> HMGFRWKLAHFRYLCQSNALPSHVKINVSRQTLFEDSFQQIMALKPYDLRRRLYVIFRGEEGLDYGGLAREWFFLLSHEVLNPMYCLFEYAGKNNYCLQINPASTINPDHLSYFCFIGRFIAMALFHGKFIDTGFSLPFYKRMLSKKLTIKDLESIDTEFYNSLIWIRDNNIEECGLEMYFSVDMEILGKVTSHDLKLGGSNILVTEENKDEYIGLMTEWRFSRGVQEQTKAFLDGFNEVVPLQWLQYFDEKELEVMLCGMQEVDLADWQRNTVYRHYTRNSKQIIWFWQFVKETDNEVRMRLLQFVTGTCRLPLGGFAELMGSNGPQKFCIEKVGKDT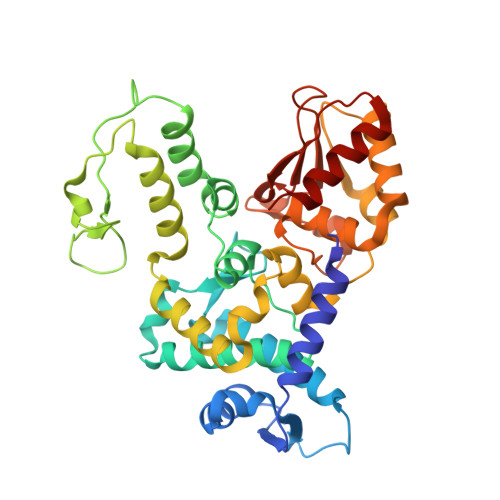WLPRSHTCFNRLDLPPYKSYEQLKEKLLFAIEETE5-(morpholin-4-ylsulfonyl)-2-{[3-(octyloxy)benzyl]oxy}benzoic 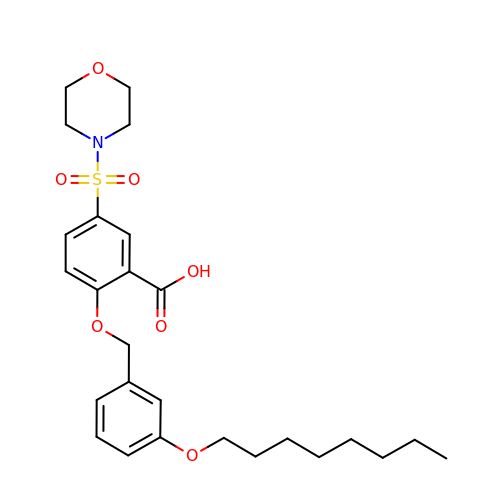acid | C26 H35 N O7 S | CMGIINZLEYERNR-UHFFFAOYSA-N>ANPCCSNPCQNRGECMSTGFDQYKCDCTRTGFYGENCTTPEFLTRIKLLLKPTPNTVHYILTHFKGVWNIVNNIPFLRSLIMKYVLTSRSYLIDSPPTYNVHYGYKSWEAFSNLSYYTRALPPVADDCPTPMGVKGNKELPDSKEVLEKVLLRREFIPDPQGSNMMFAFFAQHFTHQFFKTDHKRGPGFTRGLGHGVDLNHIYGETLDRQHKLRLFKDGKLKYQVIGGEVYPPTVKDTQVEMIYPPHIPENLQFAVGQEVFGLVPGLMMYATIWLREHNRVCDILKQEHPEWGDEQLFQTSRLILIGETIKIVIEDYVQHLSGYHFKLKFDPELLFNQQFQYQNRIASEFNTLYHWHPLLPDTFNIEDQEYSFKQFLYNNSILLEHGLTQFVESFTRQIAGRVAGGRNVPIAVQAVAKASIDQSREMKYQSLNEYRKRFSLKPYTSFEELTGEKEMAAELKALYSDIDVMELYPALLVEKPRPDAIFGETMVELGAPFSLKGLMGNPICSPQYWKPSTFGGEVGFKIINTASIQSLICNNVKGCPF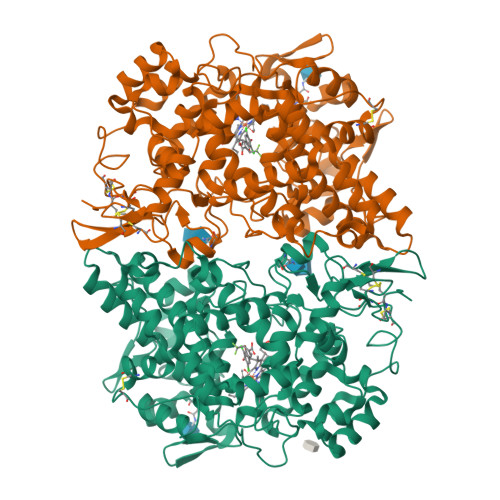TSFNVQ[4x]> MANLYVKAVPPPDMNRNTEWFMYPGVWTTYMLILFFGWLVVLSVSGCSPGMAWTVVNLAHFVVTYHSFHWMKGTPFADDQGIYNGLTWWEQMDNGQQLTRNRKFLTLVPVVLYLIASHTTDYRHPWLFLNTLAVMVLVVAKFPNMHK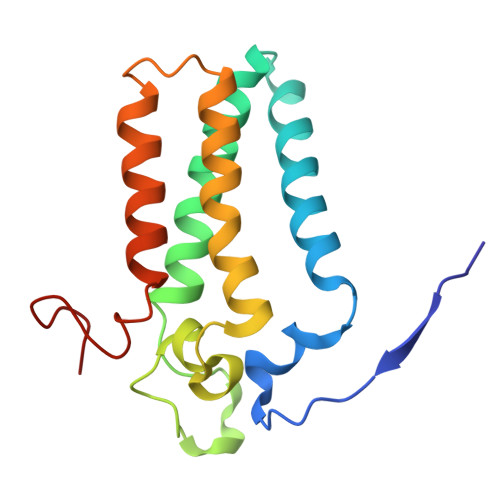VRIFGINGDK>MDHLKPEKLQTRFLNGSQNDGPRYPRCYTLTHSDSTGELFLTI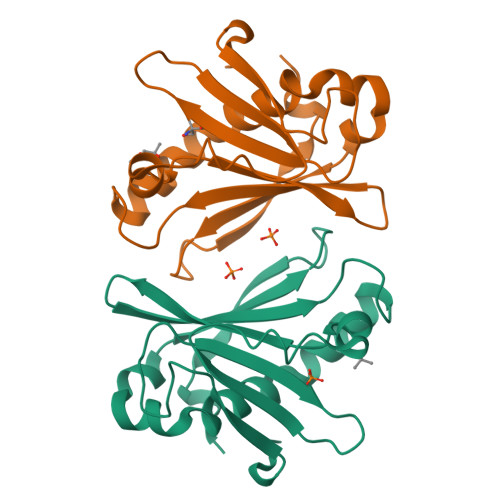GPSYDYEQISGWYTRFMRDEVLAVWEMDEEDMALHVHVHVSGGLILGSAKWRDKIFRQHMPLVLEAFRYGDRELVKKYPEMDQAPILVHFHAPNPKFDLVETWGILRDYKIEHHHHHH[2x]> MIAITGATGQLGHYVIESLMKTVPASQIVAIVRNPAKAQALAAQGITVRQADYGDEAALTSALQGVEKLLLISSSEVGQRAPQHRNVINAAKAAGVKFIAYTSLLHADTSPLGLADEHIETEKMLADSGIVYTLLRNGWYSENYLASAPAALEHGVFIGAAGDGKIASATRADYAAAAARVISEAGHEGKVYELAGDSAWTLTQLAAELTK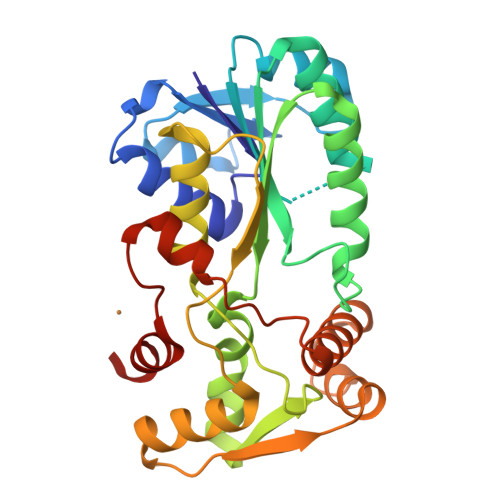QSGKQVTYQNLSEADFAAALKSVGLPDGLADMLADSDVGASKGGLFDDSKTLSKLIGHPTTTLAESVSHLFNVNN> MKELIYIEEPSILFAHGQKCTDPRDGLALFGPLNQIYGIKSGVVGTQKGLQIFKSYLDKIQKPIYNHNNITRPMFPGFEAVFGCKWESQNIVFKEITDEEIRRYLFNASTHKRTYDLVTLFNDKIITANKNDEERVDVWFVIVPEEIYKYCRPNSVLPNELVQTKSLISKSKAKSFRYTPTLFEEFNKKLKEVEKEAKTYNYDAQFHDQLKARLLEHTIPTQILRESTLAWRDFKNTFGAPIRDFSKIEGHLAWTISTAAYYKAGGKPWKLGDIRPGVCYLGLVYKKIEKSKNPQNACCAAQMFLDNGDGTVFKGEVGPWYNPEKGEYHLKPKEAKALLTQALESYKEQNKSYPKEVFIHARTRFNDEEWNAFNEVTPKNTNLVGVTITKSKPLKLYKTEGAFPIMRGNAYIVDEKKAFLWTLGFVPKLQSTLSMEVPNPIFIEINKGEAEIQQVLKDILALTKLNYNACIYADGEPVTLRFANKIGEILTASTEIKTPPLAFKYYI;> MRNKIFISHATPEDDDFTRWLSLKLIGLGYEVWCDILFLDKGVDFWSTIEKEIRENTCKFLIVSSTAGNKREGVLKELAVATKVKKHLQDDMFIIPLAIDENLSYDDINIEIVRLNAIDFKKSWAKGLQDLLDAFEKQNVPKKPPDHSKSNLLYQQIFLHDKQAIEKEETYDSNWFPIISFPNELRFHRYDWRLPKQFDVRTLAFPAIRYKEYLCTFAWEYDFIHQLPKTETYNGQESIRISTSDILSGRYDTDFIRNYECQRLIVQLINKAFELRMKDKNVREYQMSKTFAYWIEKGKLEKDKFEKIKLVGKQKNKYWHFGISAAGKLYPSPVLMVSSHIIFTMDGINLIKSKSIQHSSRRKQGKNWWNDKWREKLLAFIRFLSDDQNAIYLNVGSEEKILISNKPLKFFG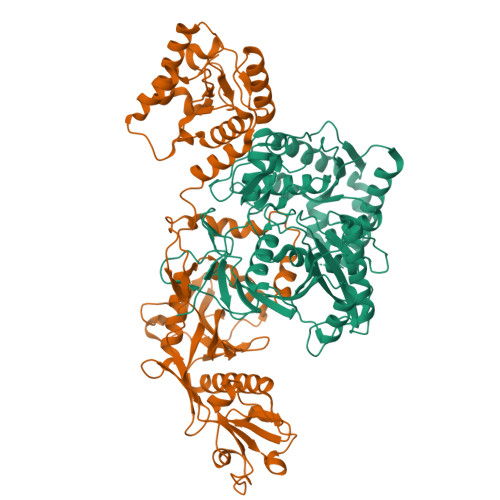KMSYVTPSEVTLEEESVLADINNFEEDTEDLDELEDIE> GLDRNRQDIGYVLGRLFAVLEKIQAEANPGLNATIADRYFGSASSTPIAVFGTLMRLLPHHLNKLEFEGRAVQLQWEIRQILEHCQRFPNHLNLE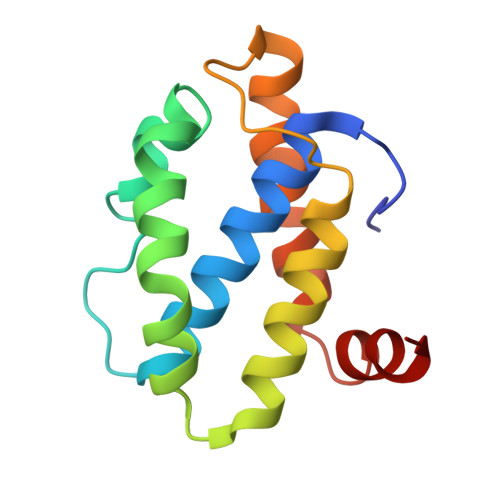QQGLFAIGYYHETQFLFTKDALKNLFNEA>[4x]MGANLNSAYAAGVKIAIVMGSKSDWATMQFAADVLTTLNVPFHVEVVSAHR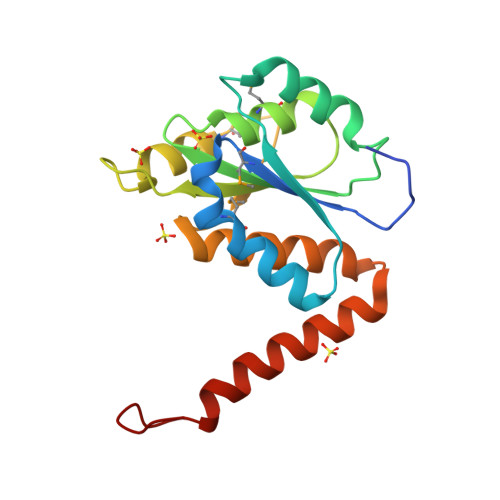TPDRLFSFAEQAEANGLHVIIAGNGGAAHLPGMLAAKTLVPVLGVPVQSAALSGVDSLYSIVQMPRGIPVGTLAIGKAGAANAALLAAQILALHDTELAGRLAHWRQSQTDDVLDNPDPREEA The Mycobacterium tuberculosis trifunctional enzyme (MtTFE) is an α2β2 tetrameric enzyme in which the α-chain harbors the 2E-enoyl-CoA hydratase (ECH) and 3S-hydroxyacyl-CoA dehydrogenase (HAD) active sites, and the β-chain provides the 3-ketoacyl-CoA thiolase (KAT) active site. Linear, medium-chain and long-chain 2E-enoyl-CoA molecules are the preferred substrates of MtTFE. Mtb is capable of switching its metabolic preference during the latent stage of infection in order to utilize host-derived fatty acids as a source of carbon rather than glucose or glycerol. The Mtb genome encodes an unusually large set of enzymes of the β-oxidation cycle; however, only a single trifunctional enzyme (MtTFE) that catalyzes three of the last four reactions in the β-oxidation cycle is present in Mtb, in contrast to other bacteria such as Escherichia coli, which has two TFEs. Here, 226 fragments were screened in a crystallographic fragment-binding study of MtTFE crystals, resulting in the structures of 16 MtTFE–fragment complexes.

The seven fragments M-10, M-49, M-76, M-79, M-80, M-92 and M-109 share a common substructure of a sulfonic acid functional group connected to an aromatic ring. The sulfonate groups of these seven fragments bind in the same region of the ECH catalytic site, but the aromatic group is bound in two different ways, such that for M-10, M-49, M-76, M-79 and M-109 it overlaps with the mode of binding of the pantetheine moiety of the substrate, whereas for M-80 and M-92 it points towards the E3 region. For one other fragment (M-10), the electron-density maps also suggested that the fragment was modified in two binding events, being a dimeric form. Of these, the structures of 12 fragments were refined to a resolution of 2.8 Å or better, two fragments to 2.9 Å resolution and two fragments to low resolutions of 3.0 and 3.2 Å, respectively. Therefore, data sets of somewhat lower resolution are also informative and these low-resolution structures were also retained for further analysis.

>MGSSHHHHHHSQDPNSMPDNTIQWDKDADGIVTLTMDDPSGSTNVMNEAYIESMGKAVDRLVAEKDSITGVVVASAKKTFFAGGDVKTMIQARPEDAGDVFNTVETIKRQLRTLETLGKPVVAAINGAALGGGLEIALACHHRIAADVKGSQLGLPEVTLGLLPGGGGVTRTVRMFGIQNAFVSVLAQGTRFKPAKAKEIGLVDELVATVEELVPAAKAWIKEELKANPDGAGVQPWDKKGYKMPGGTPSSPGLAAILPSFPSNLRKQLKGAPMPAPRAILAAAVEGAQVDFDTASRIESRYFASLVTGQVAKNMMQAFFFDLQAINAGGSRPEGIGKTPIKRIGVLGAGMMGAGIAYVSAKAGYEVVLKDVSLEAAAKGKGYSEKLEAKALERGRTTQERSDALLARITPTADAADFKGVDFVIEAVFENQELKHKVFGEIEDIVEPNAILGSNTSTLPITGLATGVKRQEDFIGIHFFSPVDKMPLVEIIKGEKTSDEALARVFDYTLAIGKTPIVVNDSRGFFTSRVIGTFVNEALAMLGEGVEPASIEQAGSQAGYPAPPLQLSDELNLELMHKIAVATRKGVEDAGGTYQPHPAEAVVEKMIELGRSGRLKGAGFYEYADGKRSGLWPGLRETFKSGSSQPPLQDMIDRMLFAEALETQKCLDEGVLTSTADANIGSIMGIGFPPWTGGSAQFIVGYSGPAGTGKAAFVARARELAAAYGDRFLPPESLLS[2x];>[2x]MSEEAFIYEAIRTPRGKQKNGSLHEVKPLSLVVGLIDELRKRHPDLDENLISDVILGCVSPVGDQGGDIARAAVLASGMPVTSGGVQLNRFCASGLEAVNTAAQKVRSGWDDLVLAGGVESMSRVPMGSDGGAMGLDPATNYDVMFVPQSIGADLIATIEGFSREDVDAYALRSQQKAAEAWSGGYFAKSVVPVRDQNGLLILDHDEHMRPDTTKEGLAKLKPAFEGLAALGGFDDVALQKYHWVEKINHVHTGGNSSGIVDGAALVMIGSAAAGKLQGLTPRARIVATATSGADPVIMLTGPTPATRKVLDRAGLTVDDIDLFELNEAFASVVLKFQKDLNIPDEKLNVNGGAIAMGHPLGATGAMILGTMVDELERRNARRALITLCIGGGMGVATIIERV> TVGCVVVDREGRCAAATSTGGLMNKMTGRIGDSPLIGAGTYACDVCGVSCTGEGEAIIRGTLAREVAAVMEYKGLKLHQAVDFVIKHRLDEGKAGLIAVSNTGEVACGFNCNGMFRACATEDGFME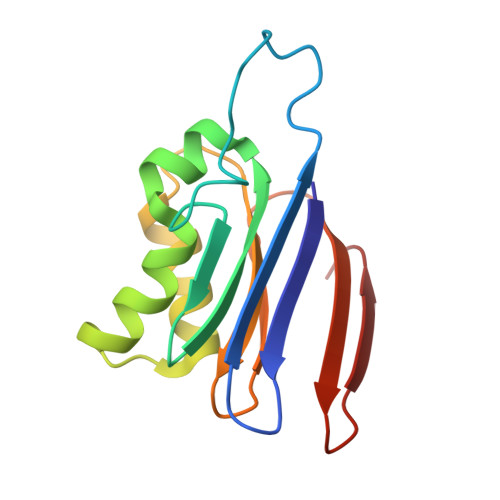VAIWD~{N}-methyl-1-[4-[[[1-methyl-5-(phenylmethyl)pyrazol-3-yl]carbonylamino]methyl]phenyl]benzimidazole-5-carboxamide | C28 H26 N6 O2 | 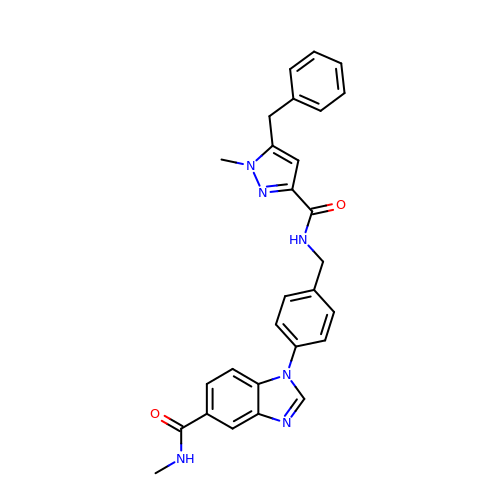OVVBAKUOCIBISQ-UHFFFAOYSA-N>[2x]PLWTWSPSASVAGTGVGVDPEYVWDEEADPVLAAVIDRGEVPAVNALLKQWTRNDQALPGGLPGDLREFMEHARRMPSWADKAALDRGAQFSKTKGIYVGALYGLGSGLMSTAIPRESRAVYYSKGGADMKDRIAKTARLGYDIGDLDAYLPHGSMIVTAVKTRMVHAAVRHLLPQSPAWSQTSGGQKIPISQADIMV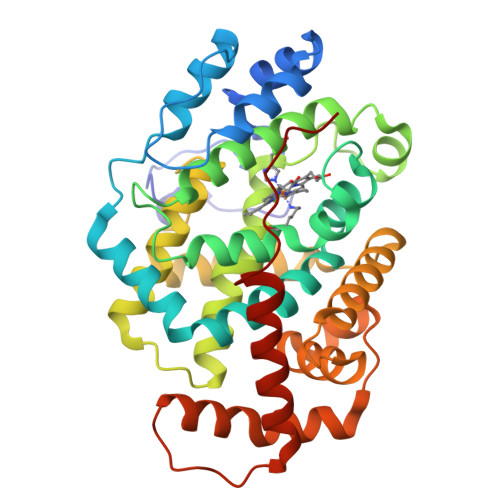TWHSLATFVMRKMKQWGVRVNTADAEAYLHVWQVSAHMLGVSDEYIPATWDAANAQSKQVLDPILAHTPEGEALTEVLLGIVAELDAGLTRPLIGAFSRYTLGGEVGDMIGLAKQPVLERLIATAWPLLVAFREGLIPLPAVPAVLWTLEEALRKFVLLFLSEGRRIAIDIPD>[2x]IREILKMGDERLLRIAQPVPSELLGSE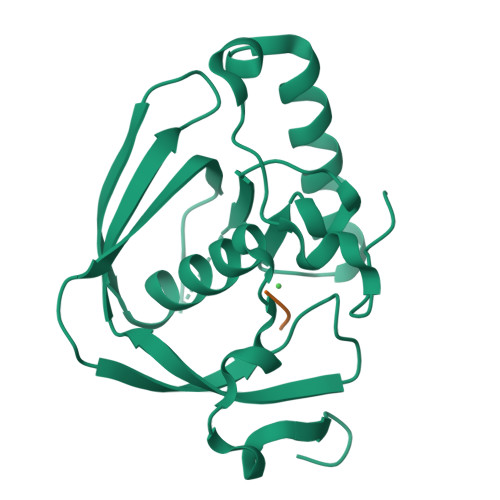ELQRLIDDMFETMHHVGGVGLAAPQIGVDLQLVIFGFERSERYPDAPAVPPTILLNPRITPLDDEMEEGWEGCLSVPGLRGAVSRHRRIRYQGLDPQGQPIDRSVEGFHARVVQHECDHLIGRLYPSRITDFSKFGFTEVLFP;> MAS Human spermine oxidase (hSMOX) plays a central role in polyamine catabolism. The second pathway involves a one-step reaction where Spm is directly oxidized by hSMOX to produce Spd, H2O2 and 3-AP. Due to its association with several pathological processes, including inflammation and cancer, hSMOX has garnered interest as a possible therapeutic target. The monomeric enzyme consists of two domains (the FAD containing F-domain and the substrate-binding S-domain) with the non-covalently bound prosthetic FAD group in an elongated conformation at the interface between the domains.

The co-crystal structure of hSMOX with JNJ-1289 was determined at 2.1 Å resolution, revealing that JNJ-1289 binds to an allosteric site, providing JNJ-1289 with a high degree of selectivity towards hSMOX. To understand the binding of JNJ-1289 to ehSMOX, the inhibitor was soaked into crystals of ehSMOX and diffraction to anisotropic resolution cutoffs of 2.98, 2.98, and 2.04 Å was collected. JNJ-1289 binds ehSMOX in an allosteric pocket ~13 Å from the FAD isoalloxazine ring. Critically, one of the loops near the active site entrance (aa 190–210), which was not resolved in the first ehSMOX structure, is now well defined and is bent in front of the substrate-binding pocket above JNJ-1289, indicating stabilization of the loop upon inhibitor binding. The electron density for JNJ-1289 allows unambiguous placement in an allosteric pocket nestled between the protein surface of the ‘open’ structure and the previously unresolved aa190–210 loop closing on top. The JNJ-1289 phenol oxygen is involved in a H-bond with the carboxylic acid of Glu207. The central thiazole is involved in several π-stacking interactions with residues Val184 (H-π), Tyr181 (T-shaped π) and Trp205 (π-π). The imidazopyridine ring of the inhibitor forms a H-bond with the carboxylic acid of Glu185, while the pyridine ring makes an edge-to-face interaction with the side chain of Tyr127. The loop position in the JNJ-1289 bound-ehSMOX confers a U-shaped substrate-binding cavity that is more similar to the zmPAOX than to the mPAOX structure. As observed in the JNJ-1289-ehSMOX co-crystal structure, the compound-induced conformation of aa190–210 closes off the putative active site.

> GGPGPRVVVIGAGLAGLAAAKALLEQGFTDVTVLEASSHIGGRVQSVKLGHATFELGATWIHGSHGNPIYHLAEANGLLEETTDGERSVGRISLYSKNGVACYLTNHGRRIPKDVVEEFSDLYNEVYNLTQEFFRHDKPVNAESQNSVGVFTREEVRNRIRNDPDDPEATKRLKLAMIQQYLKVESCESSSHSMDEVSLSAFGEWTEIPGAHHIIPSGFMRVVELLAEGIPAHVIQLGKPVRCIHWDQASGSGSGSVVVECEDCELIPADHVIVTVSLGVLKRQYTSFFRPGLPTEKVAAIHRLGIGTTDKIFLEFEEPFWGPECNSLQFVWEDEAESHTLTYPPELWYRKICGFDVLYPPERYGHVLSGWICGEEALVMETLSDEAVAEICTEMLRQFTGNPNIPKPRRILRSAWGSNPYFRGSYSYTQVGSSGADVEKLAKPLPGLQVLFSGEATHRKYYSTTHGALLSGQREAARLIEMYRDLFQQSRPRL>NDDINKGPSGDNENNGTDDNDRTAGPIITFTHDLTSDFLSSPL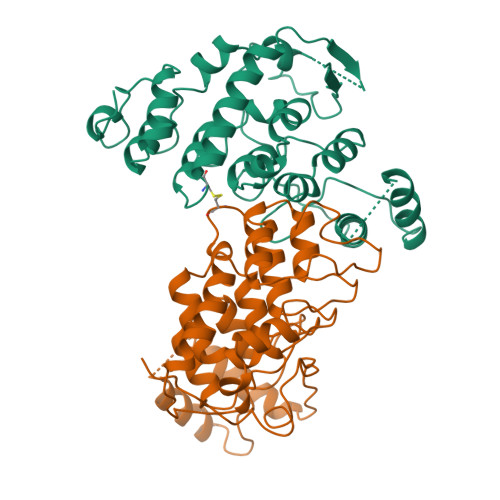KIMKALPSPVVNDNEQKMKLEAFLQRLLFPEIQEMPTSLNNDSSNRNSEGGSSNQQQQHVSFDSLLQEVNDAFPNTQLNLNIPVDEHGNTPLHWLTSIANLELVKHLVKHGSNRLYGDNMGESCLVKAVKSVNNYDSGTFEALLDYLYPCLILEDSMNRTILHHIIITSGMTGCSAAAKYYLDILMGWIVKKQNRPIQSGTNEKESKPNDKNGERKDSILENLDLKWIIANMLNAQDSNGDTCLNIAARLGNISIVDALLDYGADPFIANKSGLRPVDFGAGLE[2x]> MSQKDNLLDNPVEFLKEVRESFDIQQDVDAMKRIRHDLDVIKEESEARLKLYRSLGVILDLENDQVLINRKNDGNIDI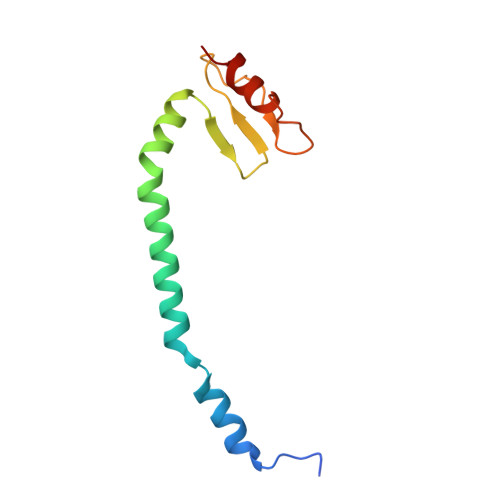LPLDNNLSDFYKTKYIWERLGK> SGFEFHGYAPSGVIMNDSGASTKSGAYITPAGETGGAI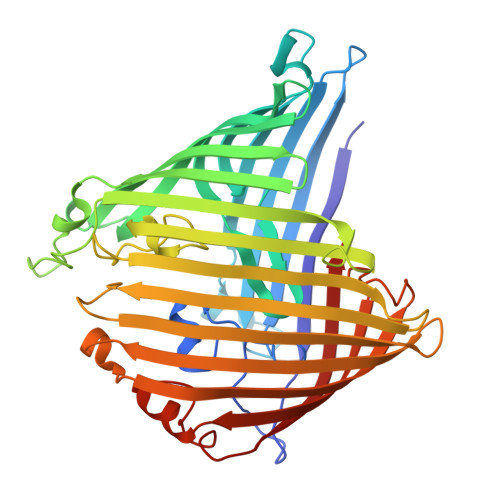GPLGNAADTYVIMNLEHKQTLDNGATTRFKVMVADGQTSYNDWTASTSDLNVLQAFVELGNLPTFAGPFKGSTLWAGKRFDRDNFAIHWILSCVVFLAGTGGGIYDVKWNDGLRSNFSLYGRNFGDIDDSSNSVQNYILTMNHFAGPLQMMVSGLRAKDNDERKDSNGNLAKGDAANTGVHALLGLHNDSFYGLRDGSSKTALLYGHGLGAEVKGIGSDGALRPGADTWRIASYGTTPLSENWSVAPAMLAQRSKDRYADGDSYQWATFNLRLIQAINQNFALAYEGSYQYMDLKPEGYNDRQAVNGSFYKLTFAPTFKVGSIGDFFSRPEIRFYTSWMDWSKKLNNYASDDALGSDGFNSGGEWSFGVQMETAF>MMSDQENENEHAKAFLGLAKCEEEVDAIEREVELYRLNKMKPVYEKRDAYIDEIAEFWKIVLSQHVSFANYIRASDFKYIDTIDKIKVEWLALESEMYDTRDFSITFHFHGIEGDFKEQQVTKVFQIKKGKDDQEDGILTSEPVPIEWPQSYDSINPDLIKDKRSPEGKKKYRQGMKTIFGWFRWTGLKPGKEFPHGDSLASLFSEEIYPFCVKYYAEAQ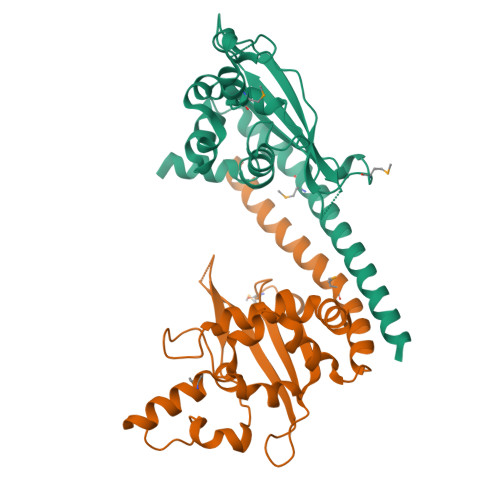RDLEDEEGESGLSADGDSEDDDGSLGEVDLPLSDEEPSS[2x]>SMKGIEKEVNVYKSEDSLGLTITDNGVGYAFIKRIKDGGVIDSVKTICVGDHIESINGENI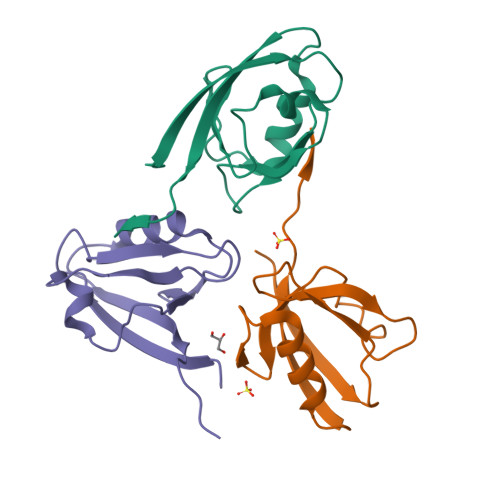VGWRHYDVAKKLKELKKEELFTMKLIEPKKSSEA[3x]>SSKEPKFTKCRSPERETFSCHWTDEVHHGTKNLGPIQLFYTRRNTQEWTQEWKECPDYVSAGENSCYFNSSFTSIWIPYCIKLTSNGGTVDEKCFSVDEIVQPDPPIALNWTLLNVSLTGIHADIQVRWEAPRNADIQKGWMVLEYELQYKEVNETKWKMMDPILTTSVPVYSLKVDKEYEVRVRSKQRNSGN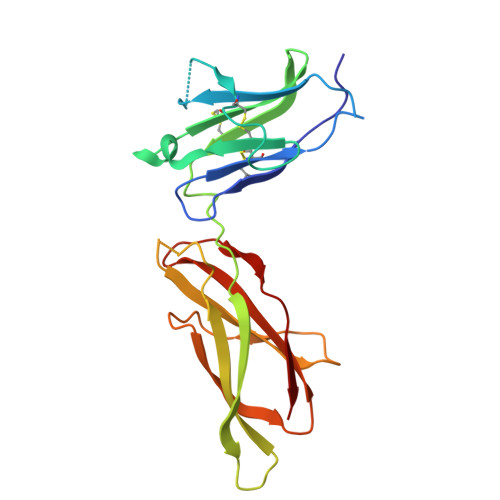YGEFSEVLYVTL[2x]> MSEQSICQARAAVMVYDDANKKWVPAGGSTGFSRVHIYHHTGNNTFRVVGR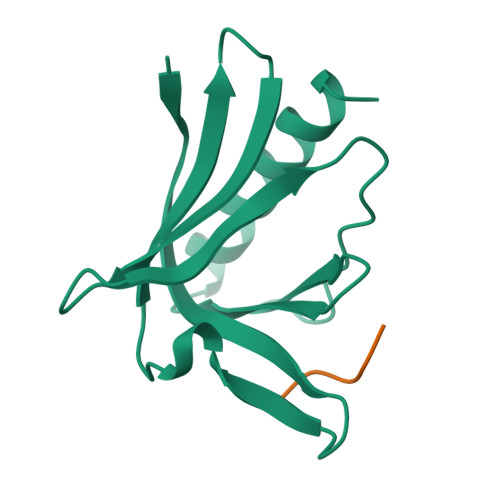KIQDHQVVINCAIPKGLKYNQATQTFHQWRDARQVYGLNFGSKEDANVFASAMMHALEVLN;> XFPPPPT>[2x]APQQINDIVHRTITPLIEQQKIPGMAVAVIYQGKPYYFTWGYADIAKKQPVTQQTLFELGSVSKTFTGVLGGDAIARGEIKLSDPTTKYWPELTAK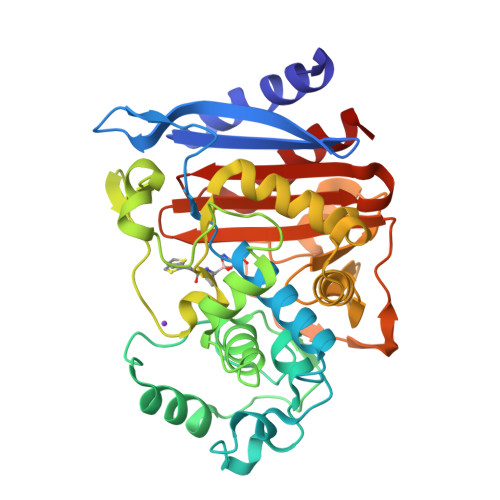QWNGITLLHLATYTAGGLPLQVPDEVKSSSDLLRFYQNWQPAWAPGTQRLYANSSIGLFGALAVKPSGLSFEQAMQTRVFQPLKLNHTWINVPPAEEKNYAWGYREGKAVHVSPGALDAEAYGVKSTIEDMARWVQSNLKPLDINEKTLQQGIQLAQSRYWQTGDMYQGLGWEMLDWPVNPDSIINGSDAKIALAARPVKAITPPTPAVRASWVHKTGATGGFGSYVAFIPEKELGIVMLANKNYPNPARVDAAWQILNALQ>[8x]GASRQRKLEALIRDPRSPINVESLLDGLNSLVLDLDFPALRKNKNIDNFLNRYEKIVKKIRGLQMKAEDYDVVKVIGRGAFGEVQLVRHKASQKVYAMKLLSKFEMIKRSDSAFFWEERDIMAFANSPWVVQLFYAFQDDRYLYMVMEYMPGGDLVNLMSNYDVPEKWAKFYTAEVVLALDAIHSMGLIHRDVKPDNMLLDKHGHLKLADFGTCMKMDETGMVHCDTAVGTPD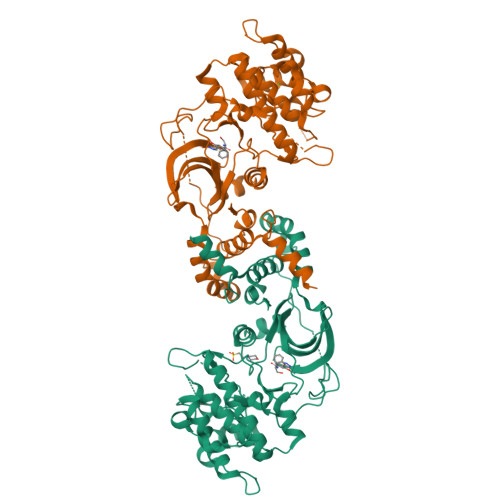YISPEVLKSQGGDGFYGRECDWWSVGVFLYEMLVGDTPFYADSLVGTYSKIMDHKNSLCFPEDAEISKHAKNLICAFLTDREVRLGRNGVEEIRQHPFFKNDQWHWDNIRETAAPVVPELSSDIDSSNFDDIEDDKGDVETFPIPKAFVGNQLPFIGFTYYR>GAMGSMATYEVLCEVAEKLGTDDREVVLFLLNVFIPQPTLAQLIGALRALKEEGRLTFPLLAECLFRAGRRDLLRDLLHLDPRFLERHLAGTMSYFSPYQLTVLHVDGELCARDIRSLIFLSKDTIGSRSTPQTFLHWVYC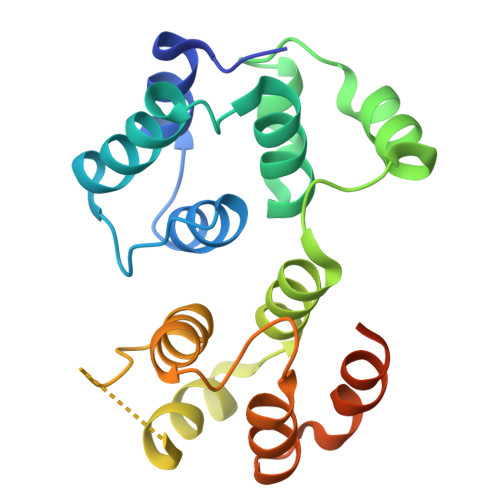MENLDLLGPTDVDALMSMLRSLSRVDLQRQVQTLMGLHLSGPSHSQHYRHTP[6x]> MAHHHHHHMNLRAAGPGWLFCPADRPERFAKAAAAADVVILDLEDGVAEAQKPAARNALRDTPLDPERTVVRINAGGTADQARDLEALAGTAYTTVMLPKAESAAQVIELAPRDVIALVETARGAVCAAEIAAADPTVGMMWGAEDLIATLGGSSSRRADGAYRDVARHVRSTILLAASAFGRLALDAVHLDILDVEGLQEEARDAAAVGFDVTVCIHPSQIPVVRKAYRPSHEKLAWARRVLAASRSERGAFAFEGQMVDSPVLTHAETMLRRAGEATSE

Mtb protein Rv2498c is currently annotated as the β-subunit (CitE) of the heterotrimeric prokaryotic citrate lyase complex involved in TCA cycle cataplerosis. Combining phylogenetic analysis, in vitro enzymatic assays, in vivo Mtb experiments, and X-ray crystallography, we identified Mtb Rv2498c as an essential stereospecific bifunctional β-hydroxyacyl-CoA lyase (β-HAC lyase) that carries out the last step of itaconate dissimilation pathway and confers resistance to itaconate. A systematic evaluation of substrate specificity revealed (R)-HMG-CoA ∼ (S)-citramalyl-CoA >>> (S)-malyl-CoA ∼ β-methylmalyl-CoA as substrates for Rv2498c. To investigate the molecular basis of Rv2498c substrate stereospecificity for the carbon–carbon bond, we determined the structures of Rv2498c in a variety of liganded states by X-ray crystallography.

Rv2498c catalyzed the carbon–carbon bond cleavage of (S)-citramalyl-CoA to form pyruvate and Ac-CoA (kcat/Km = 2.3 × 105).> MIFPKQYPIINFTTAGATVQSYTNFIRAVRGRLTVLPNCVGLPINQRFILVELSNHAELSVTLALNVCNAYVVGYRAGNSAYFFHPDNQEDAEA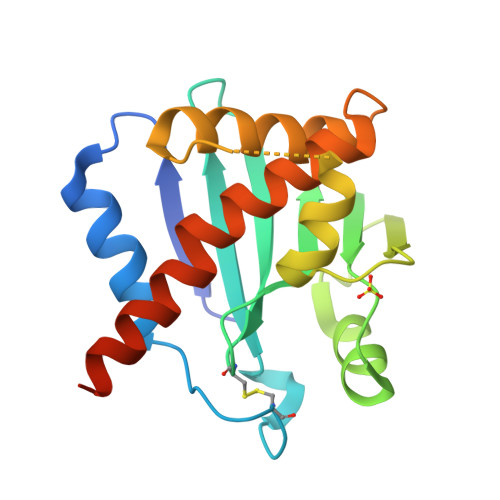ITHLFTDVQNRYTFAFGGNYDRLEQLAGNLRENIELGNGPLEEAISALYYYSTGGTQLPTLARSFIICIQMISEAARFQYIEGEMRTRIRYNRRS>[2x]SNAMRKINFSAGPSTLPLEILEQAQKELCDYQGRGYSIMEISHRTKVFEEVHFGAQEKAKKLYELNDDYEVLFLQGGASLQFAMIPMNLALNGVCEYANTGVWTKKAIKEAQILGVNVKTVASSEESNFDHIPRVEFSDNADYAYICSNNTIYGTQYQNYPKTKTPLIVDASSDFFSRKVDFSNIALFYGGVQKNAGISGL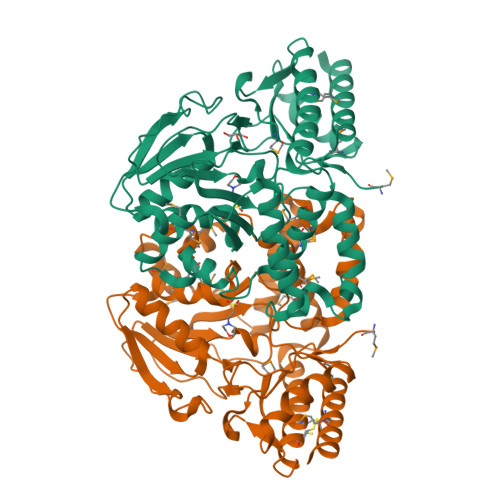SCIFIRKDMLERSKNKQIPSMLNYLTHAENQSLFNTPPTFAIYMFNLEMDWLLNQGGLDKVHEKNSQKATMLYECIDLSNGFYKGHADKKDRSLMNVSFNIAKNKDLEPLFVKEAEEAGMIGLKGHRILGGIRASIYNALNLDQVKTLCEFMKEFQGKYA> AAA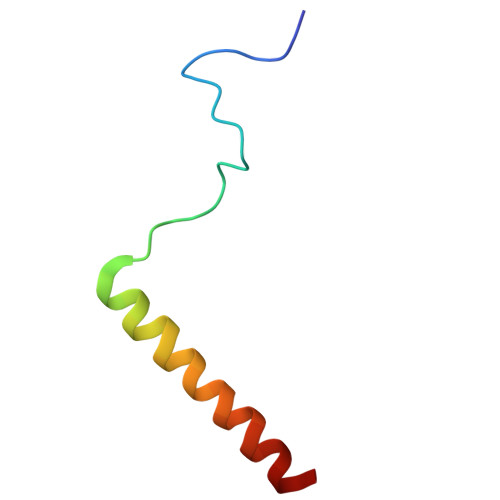AAAAAAAAAAAAAAAAAAAAAAAAAAAAAAAAAAAAAAAAAAA>[2x]ALYEDPPDQKTSPSGKPATLKICSWNVDGLRAWIKKKGLDWVKEEAPDILCLQETKCSENKLPAELQELPGLSHQYWSAPSDKEGYSGVGLLSRQAPLKVSYGIGDEEHDQEGRVIVAEFDSFVLVTAYVPDAGRGLVRLEYRQRWDEAFRKFLKGLASRKPLVLCGDLNVAHEEIDLRNPKGNKKNAGFTPQERQGFGELLQAVPLADSFRHLYPNTPYAYTFWTYMMNARSKNVGWRLDYFLLSHSLLPALCDSKIRSKALGSDHCPITLYLAL

AP sites are then processed by apurinic/apyrimidinic endonuclease 1 (APE1), which cleaves the phosphodiester DNA backbone at the 5′ end of the AP site using its endonuclease activity. Upon binding an AP site, APE1 flips the AP site out of the DNA double helix and into an extrahelical position within the compact APE1 active site. In the human APE1 substrate complex, N174 is within hydrogen bonding distance of N212 and the AP site bridging oxygen (O5) and deoxyribose sugar oxygen (O4). To assess the role of N174 during APE1 catalysis, we rationally designed four mutations of N174: N174A, N174D, N174Q, and N174K.

The APE1N174D mutant had a kobs of 0.0026 ± 0.0010 s−1, corresponding to a 330,000-fold reduction in kobs compared to APE1WT. Next, we crystallized the APE1N174D mutant protein bound to a 21-mer dsDNA oligo containing a centrally located THF AP site analog. In these crystals, the AP site has been cleaved by APE1 resulting in a product complex that diffracted to 2.10 Å resolution in the P1 space group. Within this structure, both N174D and the AP site are positioned in the active site with clear density for the cleaved DNA backbone, however there is no metal bound. We overlayed the APE1N174D mutant product complex with the APE1WT product complex and observed similar active site conformations (RMSD = 0.335 of 2321 atoms). Consistent with what we observed for the APE1N174A mutant, residue N212 in the APE1N174D mutant failed to undergo the rotameric shift observed in APE1WT following product formation. The 5′ phosphate and 3′ hydroxyl DNA termini in the APE1N174D mutant product complex are only moderately shifted compared to their positions in the APE1WT product complex. These shifts are considerably smaller than those observed in the APE1N174A mutant product complex, supporting the idea that the N174 side chain acts as a steric barrier to keep the cleaved 5′ and 3′ DNA termini within the APE1 active site. However, given that the rate of cleavage for the APE1N174D mutant is even lower than in the APE1N174A mutant, we hypothesize the charge of the N174D mutation may account for the remaining difference in cleavage rates between our mutants. We found that a larger area of the APE1N174D mutant active site surface was more negatively charged than APE1WT.>MNASDFRRRGKEMVDYMADYLEGIEGRQVYPDVQPGYLRPLIPATAPQEPDTFEDILQDVEKIIMPGVTHWHSPYFFAYFPTASSYPAMLADMLCGAIGCIGFSWAASPACTELETVMMDWLGKMLQLPEAFLAGEAGEGGGVIQGSASEATLVALLAARTKVVRRLQAASPGLTQGAVLEKLVAYASDQAHSSVERAGLIGGVKLKAIPSDGKFAMRASALQEALERDKAAGLIPFFVVATLGTTSCCSFDNLLEVGPICHEEDIWLHVDAAYAGSAFICPEFRHLLNGVEFADSFNFNPHKWLLVNFDCSAMWVKRRTDLTGAFKLDPVYLKHSHQGSGLITDYRHWQLPLGRRFRSLKMWFVFRMYGVKGLQAYIRKHVQLSHEFEAFVLQDPRFEVCAEVTLGLVCFRLKGSDGLNEALLERINSARKIHLVPCRLRGQFVLRFAICSRKVESGHVRLAWEHIRGLAAELLAAEE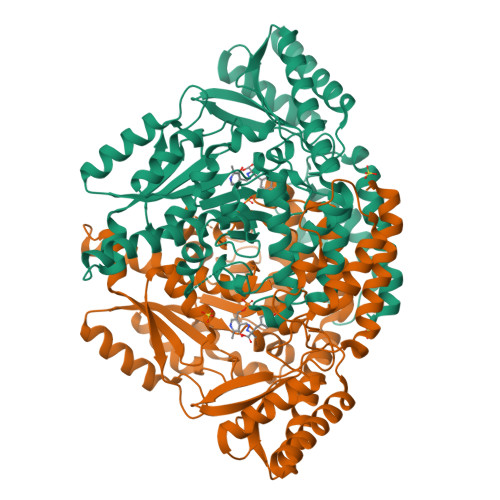GKAEIKS[2x]In this study, we extracted extracellular fibrils from lab-cultured Bacillus amyloiquefaciens, a Gram-positive bacterium with great potential in biotechnological applications such as plant growth promotion, biocontrol, and commercial enzyme production. In this study, we use cryo-EM to identify protein fibrils surrounding lab-cultured Bacillus amyloiquefaciens and discover an unreported fibril species in addition to the flagellar fibrils. In summary, our study identified two protein fibrils outside Bacillus bacteria: the extensively studied flagella and the previously undiscovered Vpr fibrils.

The amino acid sequence from the ModelAngelo model was then used to search for proteins with similar sequences, and Bacillus amyloiquefaciens Vpr, a extracellular S8 family serine peptidase, was the top hit (sequence identity 77%). Vpr proteins fold into four domains: a catalytic domain containing the typical catalytic triad of serine protease, an insert domain visible only in the cryo-EM map with a low threshold, and two assembly domains mainly responsible for inter-subunit interactions. Vpr proteins assemble into fibrils with a helical symmetry and a C2 symmetry. The fibrils are held together by two sets of inter-subunit interactions, one between subunit n and n+1 and the other between subunit n and n-2′ (the C2 symmetry counterpart of n-2). These inter-subunit interactions are predominantly hydrophilic, including hydrogen bonds and salt bridges, but there are also hydrophobic interactions. The relative position of the catalytic triad (Asp186, His230, and Ser531) suggests that the active site of Vpr protein is well folded and may be in a functional conformation. The active site in each subunit of Vpr fibrils is located in a cleft on the surface of the fibrils and is accessible to the solvent. These observations suggest that Vpr may maintain its peptidase activity when assembled into fibrils. There is an inner tunnel of ~23 Å in width at the center of Vpr fibrils, and extra densities are found inside the tunnel. The shape of the extra densities is a straight tube with an approximately circular cross-section, and the diameter of the circular cross-section is ~15 Å. These extra densities may suggest binding of unknown ligands, which should be negatively charged, as multiple lysine residues surround these densities (blue arrows).

>LKKGIIRYLLPAFVLSFTLSTSSQAAPASKPQTPDLEKAEVFGDIDMTTGKQTTVIVELKEKSLAEAKELGKAQTKSKLKSERSKVKKKALKTIKHGKINREYEQVFSGFSMKLPANEIPKLLSDQDVKAVYPNVTYHTDQLKDKDITLSKDAVSPQMDDSAPYIGANDAWKLGYTGKGVKVAIIDTGVEYKHPDLKKNFGQYKGYDFVDNDYDPEETPSGDPRGASTDHGTHVAGTVAANGTIKGVAPDATLLAYRVLGPGGSGTTENVIAGIERAVQDGADVMNLSLGNSVNNPDWATSTALDWAMSEGVTAVTSNGNSGPNNWTVGSPGTSREAISVGATQLPLNEYAVSFGSYSSAKVMGYNKEDDIKALNKKETELIEAGIGEQKDFEGKDLKGKVAVVKRGSIAFVDKADNAKKAGAIGMVVYNNAPGEIEANVPGMSVPTVKLSSEDGEKLVSQLKAGGTKATFHLSVAKSLTEQMADFSSRGPVMDTWMIKPDVSAPGVNIVSTIPTHDPADPYGYGSKQGTSMASPHVAGAAAVIKQAKPKWSPEQIKAALMNTAETLTDADGDVYPHNAQGAGSIRIMKAIKADSLVAPGSYSYGTFMKDKGNETKKETFTIENQSSIRKSYQLEYSFNGTGITVSGTDRVVIPAHQTGKVNAKVKVNAKKVKAGTYEGTVTVREGGKTVAKVPTLLIVKEPDYPRVTSIDVQDGTTQGTYQIETYLPAGAEELAFLVYDSNLDFVGQAGIYKKQDKGYQYFDWNGKVNGDTALPAGEYYMLAYAANKGKSSQVLTEKPFIIE[18x]> ESKKRQWALEDFEIGRPLGKGKFGNVYLAREKQSKFILALKVLFKAQLEKAGVEHQLRREVEIQSHLRHPNILRLYGYFHDATRVYLILEYAPLGTVYRELQKLSKFDEQRTATYITELANALSYCHSKRVIHRDIKPENLLLGSAGELKIADFGWSVHAPSSRRTTLCGTLDYLPPEMIEGRMHDEKVDLWSLGVLCYEFLVGKPPF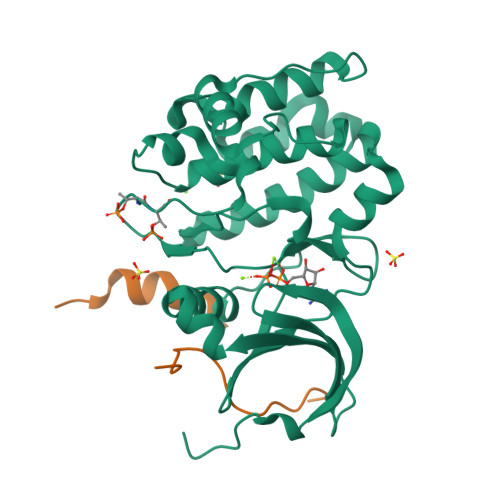EANTYQETYKRISRVEFTFPDFVTEGARDLISRLLKHNPSQRPMLREVLEHPWITANSSKPSNCQNKESASKQS;> MAQVKSSYSYDAPSDFINFSSLDDEGDTQNIDSWFEEKANLEN Here we determined that the arbitrium system in Bacillus subtilis phage phi3T modulates the bacterial toxin–antitoxin system MazE–MazF to regulate the phage life cycle. AimX also inhibits the function of phi3T_93, a protein that promotes lysogeny by binding to MazE and releasing MazF. In all structures, phi3T_93 shows an identical all-helices fold composed of a longer N-terminal helix (α1), followed by two shorter helices (α2 and α3) connected by a long unstructured loop forming a V-like shape. The α1 helices of two phi3T_93 monomers interact, resulting in a W-shaped tight and globular dimer that displays two shallow grooves, one across each side of the dimer molecule.

Our in silico complexes indicate that the AimX M14 residue plays an essential role in phi3T_93 and MazF recognition and substituting for a charged residue in that position should prevent AimX function. Next, we produced phi3T_93L23D by replacing a hydrophobic residue that interacts with the AimX M14 for a negatively charged one. The new charged residue had no impact on the protein integrity and quaternary organization as confirmed by solving its crystal structure and SEC analyses. BLI analysis showed no binding of phi3T_93L23D to AimX and a strong reduction (two orders of magnitude) in its affinity for MazE. Overexpression in the recipient cell of phi3T_93, but not of the phi3T_93L23D, restored the ability of the evolved phage to produce lysogens. This confirmed that phi3T_93–AimX interactions are important for the lysis–lysogeny decision. In addition, strains expressing phi3T_93, unlike those expressing phi3T_93L23D, blocked the lytic cycle and promoted lysogeny of the wt phi3T (measured by plaque and colony counts 3 h after infection). These results validate both the structural complexes and the common mechanism of recognition observed for AimX–phi3T_93 and MazE–MazF, which are driven mainly by the insertion of a hydrophobic helix into the grooves of the dimers of phi3T_93 and MazF.

>[2x]SMTNNKYYTEENKKKVWKKHMIVDKFLEQPGISEAYLNYLQEEIHNDEWIGFENEFFEELTGKPVINVGDKIKATKQYSAVH>MAKVGEGKYREDFQMDEGEDPSLLFQSYLDNVGVQIVRQIRSGERFLKIWSQTVEEIISYVAVNFPNPPGKSSEDKSTQTTGRELKKETTPTPSQRESQSSKARMAAQTASGPPALEWSATNEEDDLSVEAEIAHQIAESFSKKYKFPSRSSGILLYNFEQLKMNLDDIVKEAKNVPGVTRLARDGSKLPLRCVLGWVALANSKKF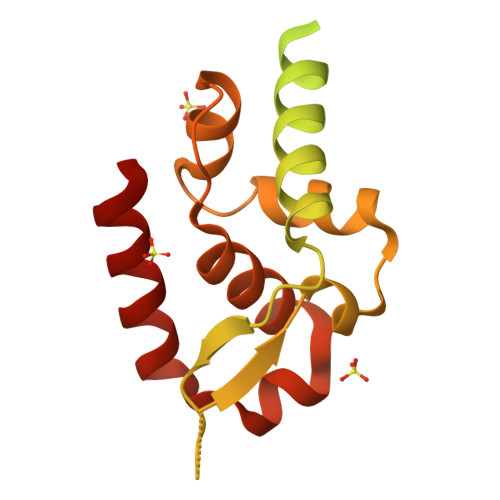QLLVESNKLSKIMQDDLNRYTSC[2x]> MGSSHHHHHHSQDPMDIKINGIKKYTIHVLAKVSASGMEFTQEKDFEHQLLLTDMLETVIRKSVEVNPVLHFHLRKSIIMNHSYFILGLNYIPPAFATKNVKSIHEIYQAIQDVNDLQLLDEFEKSKEKLINKIQQYKHSDSHSGSIRLKDRLFADKKYGSDRLGNFEKM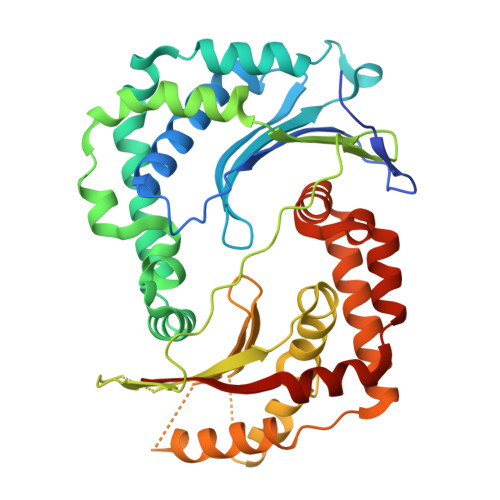NKITDNIIYAAPDMVNKICEGDGLFYHINDGAIHISNIKDFNYYIPAVINEGVEDIRTDFSKEYSILTCAYTFEHVTDLEREILIPMFDGYIGKYGHSVLFKTLRLVDENLYHISSHYDQESNLLFITVLCSKNQLSTILTKIQHTIESIEFDSVSFSLSKVMFENESRFRFEDINGLLSHVIKQHGEYKNPESFLKAIQNTDIADFYRLKANMRWVGTSIVEGG4-{[4-{[(1R,2R)-2-(dimethylamino)cyclopentyl]amino}-5-(trifluoromethyl)pyrimidin-2-yl]amino}-N-methylbenzenesulfonamide 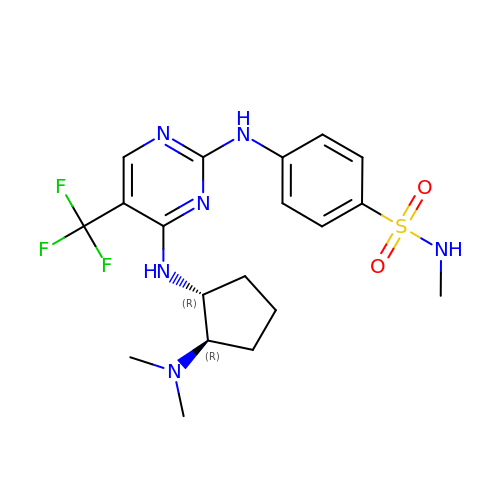| C19 H25 F3 N6 O2 S | CAUFYHKGKDJMQG-HZPDHXFCSA-N>MGSSHHHHHHSQDPDIQLLFSGFSKTRENLAVVDELLTYWNLDESESILDELEEVLLVSDFGPKTALKIVDTIRKDILAGRLKSGPQIKEALKKNIFKLLTERVT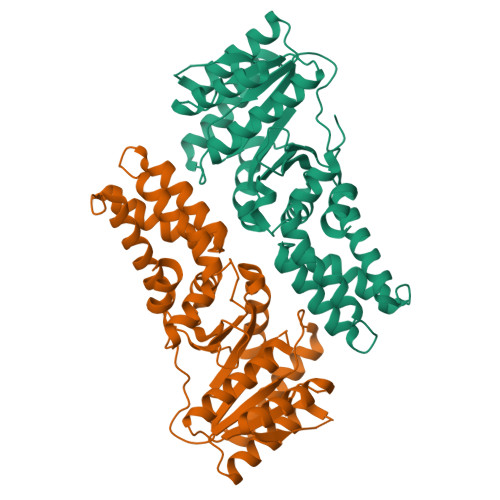TTELQLGNSRPAVLMIVGVNGGGKTTTLGKLANRFKKEGVKVLMAAGDTFRAAAGEQLEVWAQRTGSEIVMAEGPKPRPAAVLSQAVRRAVEEDFDVVLCDTSGRLHTNYNLMEELRGCKRAVSKALSSAPNEVLLVLDGTTGLNMLAQAREFNQVIGVTGFILTKLDGTARGGCVVSVVDELSIPVKFVGVGEGIDDLQPFDAQSFVDALFP[2x]>GMKSLHRPDLYSWSTFNPARNIDFNGFAWIRPEGNILIDPVALSNHDWKHLESLGGVVWIVLTNSDHVRSAKEIADQTYTKIAGPVAEKENFPIYCDRWLSDGDELVPGLKVMELQGSKTPGELALLLEET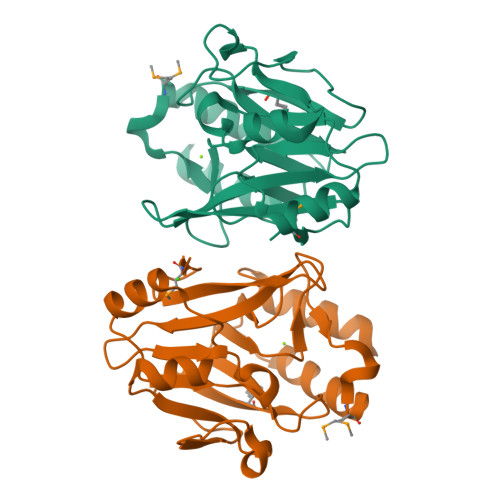TLITGDLVRAYRAGGLEILPDEKLMNKQKVVASVRRLAALEKVEAVLVGDGWSVFRDGRDRLKELVATLA[2x]>[4x]MPLTPNDIHNKTFTKSA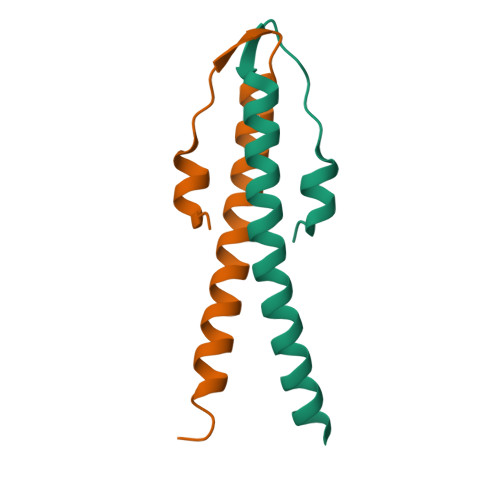RGYDEDEVNEFLAQVRKDYEIVLRKKTELEAKVNELDERI>GIHLGELGLLPSTVLAIGYFENLVNIICESLNMLPKLEVSGKEYKKFKFTIVIPKDLDANIKKRAKIYFKQKSLIEIEIPTSSRNYPIHIQFDENSTDDILHLYDMPTTIGGIDKAIEMFMRKGHIGKTDQQKLLEERELRNFKTTLENLIATDAFAKEMVEVIIEE[2x]

During phage infection, bacterial STING sense c-di-GMP generated by the CD-NTase (cGAS/DncV-like nucleotidyltransferase) encoded in the same operon and signal suicide commitment as a defense strategy that restricts phage propagation. The structure of MySTING was then solved by MR using the refined model of PcSTING. Both PcSTING and MySTING crystals contained two nearly identical protomers with root-mean-square deviations (RMSDs) of 0.29 Å and 0.64 Å for 158 and 160 matched Cα pairs in the asymmetric unit, forming canonical V-shaped dimers of STING domain. Here, our structures demonstrate that the symmetric recognition of single c-di-GMP by dimeric bacterial STING proteins is dictated by the guanidinium group of arginine residue (R233/R230 in PcSTING/MySTING) that recognizes the O6 and N7 atoms of guanine base, the backbone oxygen and amide group (H238/H235 in PcSTING/MySTING) that form three hydrogen bonds to the Watson-Crick edge of guanine base and the aspartate residue (D252/D251 in PcSTING/MySTING) that binds to the N2 atom of guanine base.

Although no nucleotide was included in the crystallization solution, the strong electron-density unambiguously identified the bound CDN as c-di-GMP. Therefore, it is clear that the four-layer stacking interaction mediated by the binding motif (Phe/Leu)/Gua/(Tyr/Phe)/Arg (e.g., F171/Gua/Y235/R233 in PcSTING or L169/Gua/Y232/R230 in MySTING), together with the arginine residue (R233/R230 in PcSTING/MySTING) that recognizes the Hoogsteen edge of the guanine base, and the aspartate residue (D252/D251 in PcSTING/MySTING) that contacts the N2 position of the guanine base contributes to the stringent specificity for c-di-GMP by bacterial STING proteins. Specificity for the symmetric [3’-5’, 3’-5’] phosphodiester bond linkage of 3’3’-c-di-GMP of bacteria STING is achieved by the side chain of conserved Thr residues (T255/T254 in PcSTING/MySTING), Asn residues (N168 in MySTING) and the main-chain of I256/T255 in PcSTING/MySTING that form hydrogen bonds with phosphate backbone and the free 2’-OH of the ribose within c-di-GMP. Changing Y232 to arginine in MySTING indeed reduced the binding affinity to c-di-GMP by nearly 1200-fold in comparison with the wild-type protein. Indeed, the ITC experiments demonstrated that the binding affinity of 3’3’-cGMAP to MySTING is about 127-fold weaker than that of c-di-GMP. Furthermore, changing c-di-GMP to c-di-AMP completely aborted the interaction with MySTING. A similar arrangement of dimers along the a axis of MySTING crystal suggests a common mode of dimer–dimer interaction. For example, the salt-bridging K209 and D300 (equivalent to K212 and D301 in PcSTING) together with E175 or an additional N171 contribute two or three ionic bonds that strengthen the filament formation of MySTING.> KTTISVIKADIGSLAGHHIVHPDTMAAANKVLASAKEQGIILDYYITHVGDDLQLIMTHTRGELDTKVHETAWNAFKEAAKVAKDLGLYAAGQDLLSDSFSG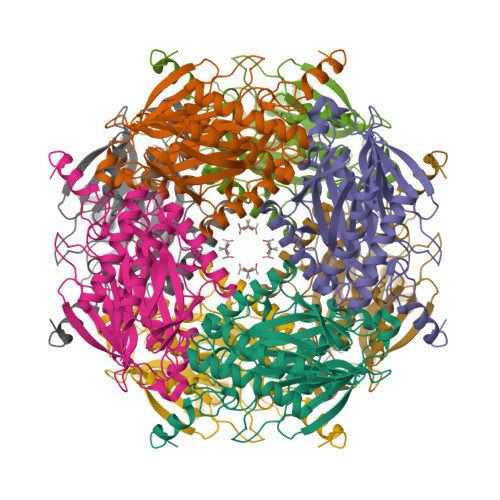NVRGLGPGVAEMEIEERASEPIAIFMADKTEPGAYNLPLYKMFADPFNTPGLVIDPTMHGGFKFEVLDVYQGEAVMLSAPQEIYDLLALIGTPARYVIRRVYRNEDNLLAAVVSIERLNLIAGKYVGKDDPVMIVRLQHGLPALGEALEAFAFPHLVPGWMRGSHYGPLMPVSQRDAKATRFDGPPRLLGLGFNVKNGRLVGPTDLFDDPAFDETRRLANIVADYMRRHGPFMPHRLEPTEMEYTTLPLILEKLKDRFKK>[2x]GAMAEYEIDEITFHKRLGILLTSWKNEEDGKTLFQDCDSILVTVGAHDDTNPYQKSTALHTWLLGYEFPSTLI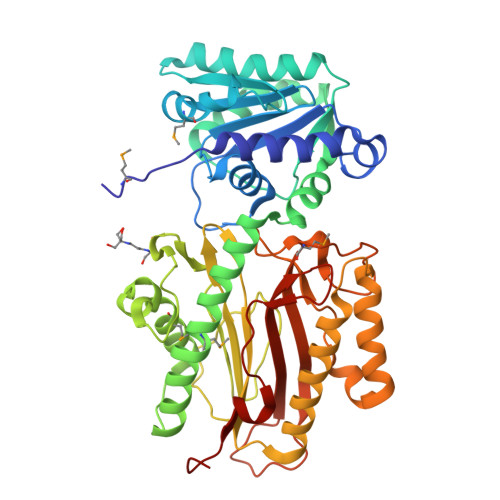LLEKHRITILTSVNKANMLTKLAETKGAAADVNILKRTKDAEENKKLFEKIIEYIRATNKKVGVFPKDKTQGKFINEWDSIFEPVKSEFNLVDASLGLAKCLAIKDEQELANIKGASRVSVAVMSKYFVDELSTYIDQGKKITHSKFSDQMESLIDNEAFFQTKSLKLGDIDLDQLEWCYTPIIQSGGSYDLKPSAITDDRNLHGDVVLCSLGFRYKSYCSNVGRTYLFDPDSEQQKNYSFLVALQKKLFEYCRDGAVIGDIYTKILGLIRAKRPDLEPNFVRNLGAGIGIEFRESSLLVNAKNPRVLQAGMTLNLSIGFGNLINPHPKNSQSKEYALLLIDTIQITRSDPIVFTDSPKAQGDISYFFGED> VDCSEYPKPACTLEYRPLCGSDNKTYAN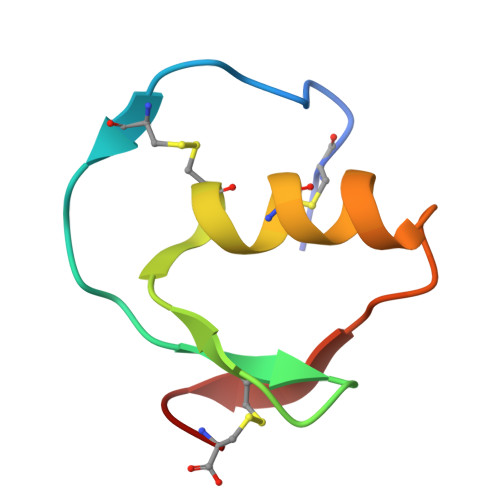KCNFCNAVVESNGTLTLSHFGKC> MAGFWVGTAPLVAAGRRGRWPPQQLMLSAALRTLKHVLYYSRQCLMVSRNLGSVGYDPNEKTFDKILVANRGEIACRVIRTCKKMGIKTVAIHSDVDASSVH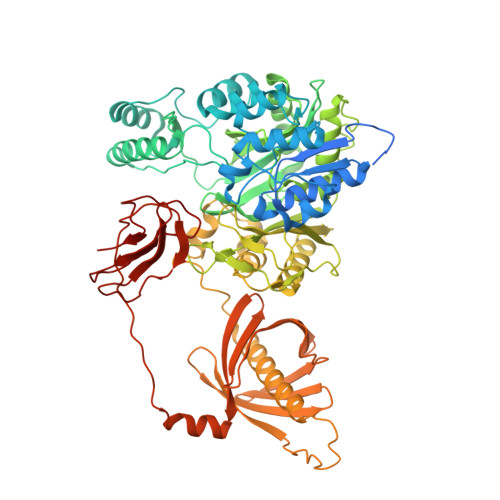VKMADEAVCVGPAPTSKSYLNMDAIMEAIKKTRAQAVHPGYGFLSENKEFARCLAAEDVVFIGPDTHAIQAMGDKIESKLLAKKAEVNTIPGFDGVVKDAEEAVRIAREIGYPVMIKASAGGGGKGMRIAWDDEETRDGFRLSSQEAASSFGDDRLLIEKFIDNPRHIEIQVLGDKHGNALWLNERECSIQRRNQKVVEEAPSIFLDAETRRAMGEQAVALARAVKYSSAGTVEFLVDSKKNFYFLEMNTRLQVEHPVTECITGLDLVQEMIRVAKGYPLRHKQADIRINGWAVECRVYAEDPYKSFGLPSIGRLSQYQEPLHLPGVRVDSGIQPGSDISIYYDPMISKLITYGSDRTEALKRMADALDNYVIRGVTHNIALLREVIINSRFVKGDISTKFLSDVYPDGFKGHMLTKSEKNQLLAIASSLFVAFQLRAQHFQENSRMPVIKPDIANWELSVKLHDKVHTVVASNNGSVFSVEVDGSKLNVTSTWNLASPLLSVSVDGTQRTVQCLSREAGGNMSIQFLGTVYKVNILTRLAAELNKFMLEKVTEDTSSVLRSPMPGVVVAVSVKPGDAVAEGQEICVIEAMKMQNSMTAGKTGTVKSVHCQAGDTVGEGDLLVELE6,7,8,9-TETRAHYDROXY-5-METHYLCARBOXAMIDO-4-OXONONANOIC ACID | C11 H19 N O8 | 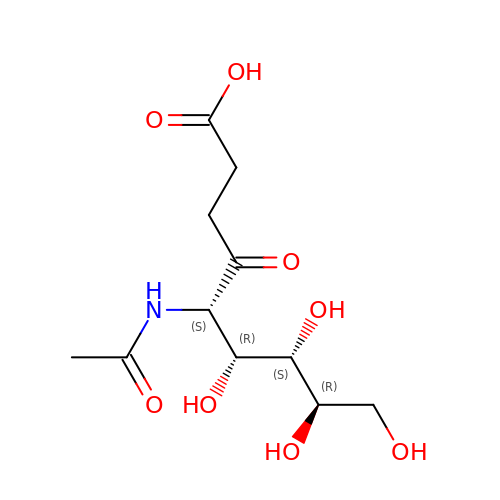IZVFSUJQAOHESA-QCNRFFRDSA-N> AGVMTGAKFTQIQFGMTRQQVLDIAGAENCETGGSFGDSIHCRGHAAGDYYAYATFGFTSAAADAKV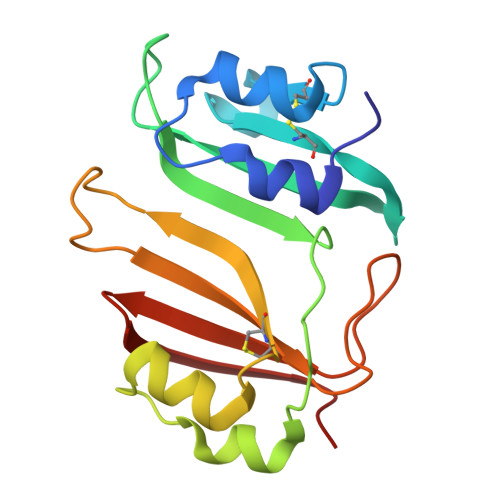DSKSQMKLLAPSAPTLTLAKFNQVTVGMTRAQVLATVGQGSCTTWSEYYPAYPSTAGVTLSLKCFDVDGYSSTGFYRGMAHLWFTDGVLQGKRQWDLV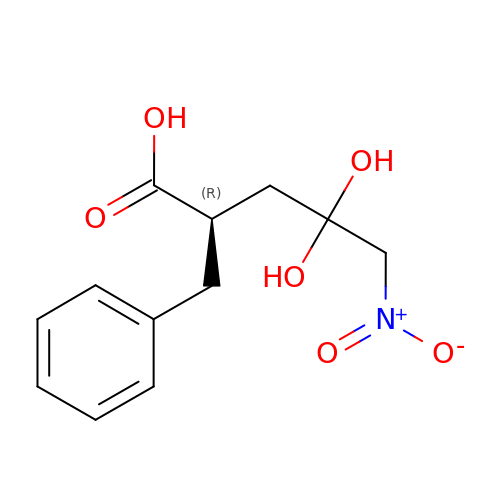(2R)-4,4-dihydroxy-5-nitro-2-(phenylmethyl)pentanoic acid | C12 H15 N O6 | CGGNZMVODZPHHK-SNVBAGLBSA-N>MATVQPIVNSHLSELDEDVFHHFGFTTKSFDFKEKFGDVKFVCVCGSSGRIHNFAISMAKLAGLALPV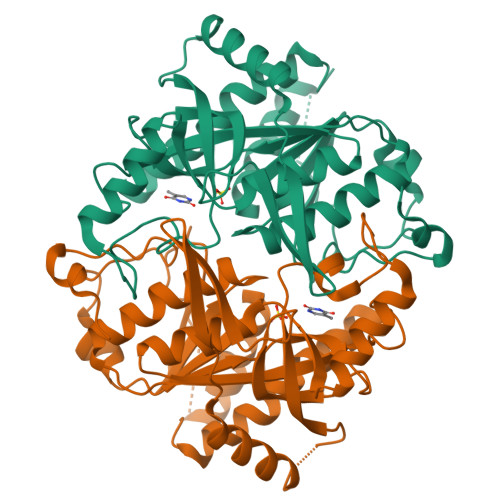ENIAGSHARFVLYKVDHILFADHGMGIPSALIMLHEVTKLLHYAGCKDVLFIRLGTSGGLGVKPGTIVLSDRCVNTKLEPYNELCILGKPVRRQTIVDLNTVNELKKLSENLSLECSVVVGGTIAANDFYEEQGRLDGSICTFSKEEKLAFLQSAYEHGIRNMEMEGTAITSHCYLTGHRAILVCVTAVNRLEGDQITISTDEFTLFAQRPGQLVGEYLKRNNGIIVR[2x]> GMSLANQIDQFLGTIMQFAENKHEILLGKAESDVKLTSTQEAILMLLAEQISTNAKIAEKLKISPAAVTKALKKLQEQELIKSSRATNDERVVLW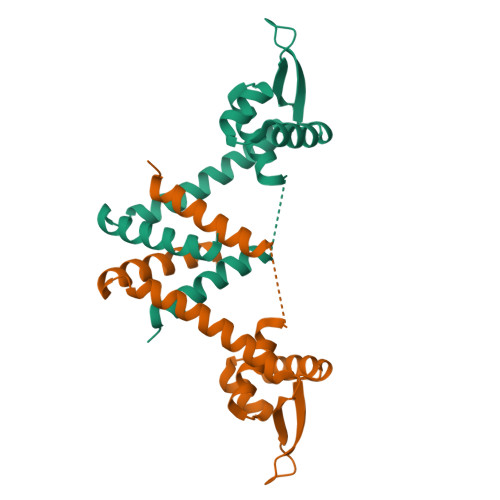SLTEKAVPVAKEHATHHEKTLSTYQELGNKFTDEEQEVISKFLSALTEEFQ> PTEFLYTSKIAAISWAATGGRQQRVYFQDLNGKIREAQRGGDNPWTGGSSQNVIGEAKLFSPLAAVTWKSAQGIQIRVYCVNKDNILSEFVYDGSKWITGQLGSVGVKVGSNSKLAALQWGGSESAPPNIRVYYQKSNGSGSSIHEYVWSGKWTAGASFGSTVPGTGIGATAIGPGRLRIYYQATDNKIREHCWDSNSWYVGGFSASASAGVSIAAISWGSTPQIRVYWQKGREELYEAAYGGSWNTPGQIKDASRPTPSLPDTFIAANSSGNIDI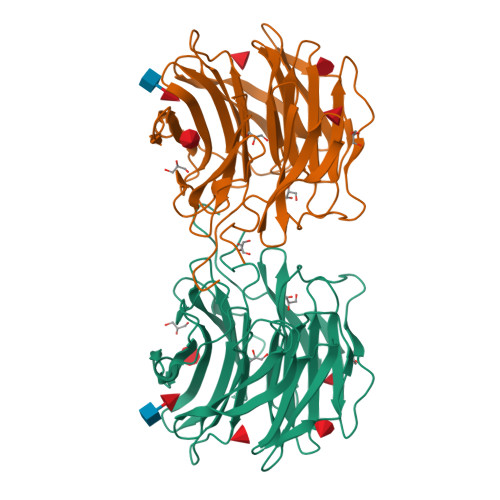SVFFQASGVSLQQWQWISGKGWSIGAVVPTGTPAGWLEHHHHHHHHHH>GSHMASMDFKTVMQELEALGKERTKKIYISNGAHEPVFGVATGAMKPIAKKIKLNQELAEELYATGNYDAMYFAGIIADPKAMSESDFDRWIDGAYFYMLSDYVVAVTLSESNIAQDVADKWIASGDELKMSAGWSCYCWLLGNRKDNAFSESKISDMLEMVKDTIHHSPERTKSAMNNFLNTVAISYVPLHEKAVEIAKEVGIVEVKRDNKKSSLLNASESI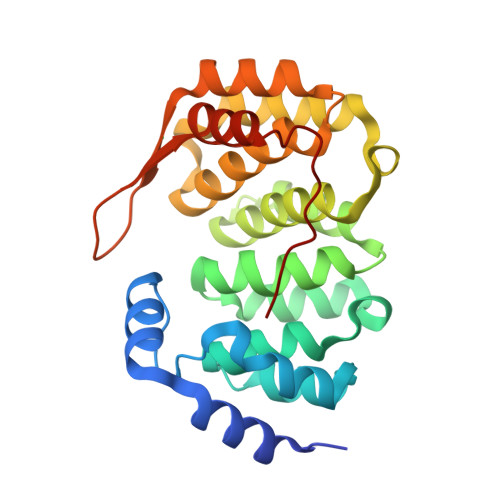QKELDRGRLGFKRKYVRC[2x]4-nitrophenyl alpha-D-glucopyranoside | C12 H15 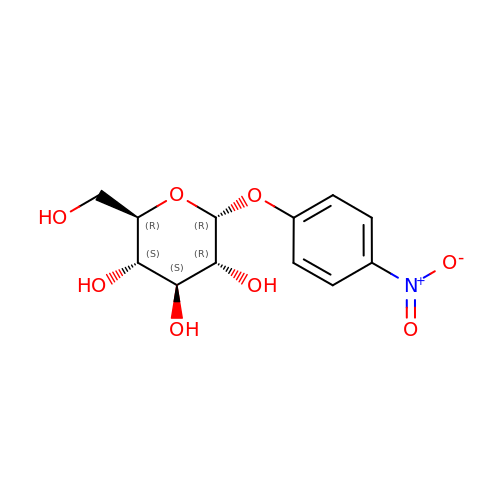N O8 | IFBHRQDFSNCLOZ-ZIQFBCGOSA-N>SNKVGTLQAQVEATQKQKAQPIDANRKYDYKLQYYLNDYVYAYFTLPQEGDKQQAQVEHLNSFYNFVPDVKAQGQVRNPSTLLDSQLVTVEGKVATYKVKYKEMIQHDKDTEEKELVTGFNIPFDEKEGKYYVSGLPWFSCIESSQAGYFSEDDQLQLTANDHVSDSQHKKVEKFLKVFFTNYTTNQDNLNLIAKNVAIVCNTTFKTIDYTYLKKDRADLIAYVQATFEVGGTTHSENFTFTLSEKDKSYYVTKLEHTIPLNYANDKD[3x]

The main model of our study is OrfG, the sole VirB8-like protein of the conjugative and integrative element ICESt3 found in the Gram-positive bacterium Streptococcus thermophilus. Bioinformatic analysis using constrained consensus TOPology prediction (CCTOP) predicted that OrfG consists of a single transmembrane α helix (residues 37 to 57) followed by a large soluble domain (OrfG64–331). This soluble region comprises two NTF2-like domains OrfG64–204 and OrfG223–331 (referred to hereafter as D1 and D2, respectively). Our data confirm that VirB8-like proteins are predominantly extracellular components, assembling into a conserved pattern, which serves as a building block of the DNA translocation channel.

To confirm this hypothesis, we used a cysteine cross-linking approach to investigate the ability of OrfGExt to form trimers in vitro. We introduced cysteines to replace facing residues at the interface D1:D1′ (K90C-E154C and Y91C-V153C) or at the interface D1:D2′ (K134C-D272C and A204C-A264C). Notably, under nonreducing conditions, variants with double-cysteine mutations, particularly OrfGExt-A204C-A264C, assemble into high-order complexes (HOC) (>100 kDa), possibly corresponding to trimeric form (theoretical molecular weight of 93 kDa). To confirm that the trimeric complex obtained using cysteine cross-linking conserved the same structural arrangement as OrfGExt, we solved the structure of OrfGExt-A204C-A264C at 2.6-Å resolution. OrfGExt-A204C-A264C shares all the characteristics of the WT structure. Despite various measurements carried out to characterize the trimers and comparing them, we observed little adaptation to the constraints brought by the disulfide bridges and/or the change of the crystallization conditions, the overall arrangement remains unchanged, as anticipated. SEC-MALS analysis conducted on both purified proteins revealed that OrfG-A204C-A264C mainly assembles into trimers (right), in contrast to the full-length OrfG, found as monomers (left). To test the potential of OrfG to function as trimer in a biological context, a orfG knockout mutant strain producing a full-length OrfG harboring the dual cysteine substitutions (A204C and A264C) was generated and subsequently examined for the presence of multimeric complexes. Mating experiments demonstrated that the strain producing the dual cysteine mutant conjugates at frequencies comparable to that of the WT strain. In the absence of DTT, the OrfG-A204C-A2064C membrane sample displayed high molecular weight complexes including one of approximatively 130 kDa, consistent with the expected size of OrfG trimers (40 kDa × 3 = 120 kDa).> MTEYKIKATIEASVAKFKRQIDSAVKSVQRFKRVADQTKDVELNANDKKLQKTIKVAKKSLDAFSNKNVKAKLDASIQDLQQKILESNFELDKLNSKEASPEVKLQKQKLTKDIAEAENKLSELEKKRVNIDVNADNSKFNRVLKVSKASLEALNRSKAKAILDVDNSVANSKIKRTKEELKSIPNKTRSRLDVDTRLSIPTIYAFKKSLDALPNKKTTKVDVDTNGLKKVYAYIIKANDNFQRQMGNLANMFRVFGTVGSNMVGGLLTSSFSILIPVIASVVPVVFALLNAIKVLTGGVLALGGAVAIAGAGFVAFGAMAISAIKMLNDGTLQASSATNEYKKALDGVKSAWTDIIKQNQSAIFTTLANGLNTVKTAMQSLQPFFSGISRGMEEASQSVLKWAENSSVASRFFNMMNTTGVSVFNKLLSAAGGFGDGLVNVFTQLAPLFQWSADWLDRLGQSFSNWANSAAGENSITRFIEYTKTNLPIIGNIFKNVFAGINNLMNAFSGSSTGIFQSLEQMTAKFREWSEQVGQSQGFKDFVSYIQTNGPLIMQLIGNIARGLVAFATAMAPIASAVLRVAVA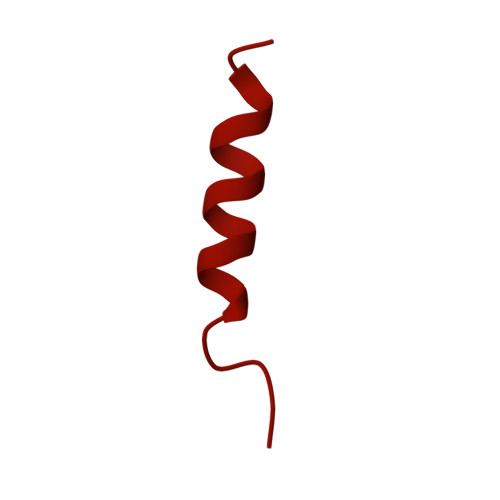ITGWIANLFEAHPATAQLVGVIITLVGAFRFLIAPILAVMDFLGPLAARLVALVTKFGWAKTGTLVLSKAMTSLKGPIKLVTAIFQLLFGKIGLIRNAITGLVTVFGILGGPITIVIGVIAALIAIFVLLWNKNEGFRNFIINAWNAIKTFMVNVWNVLKAVASVVWNAILTAITTAVSNVYNFIMIVWNQIVAYLQGLWNGIIAIATTVWNLLVTIITTVFTTIMTIVMTIWTAIWTFLSTIWNTIITIATTIWNLLVTVITTVFTTIMTIAMTIWNAIWTFLQTLWNTIVTVATKVWNAITTAISTALQAAWSFISNIWNTIWSFLSGILTTIWNKVVSIFTQVVSTISDKMSQAWNFIVTKGMQWVSTITSTLINFVNRVIQGFVNVVNKVSQGMTNAVNKIKSFIGDFVSAGADMIRGLIRGIGQMAGQLVDAAKNVAKKALDAAKSALGIHSPSREFMDVGMYSMLGFVKGIDNHSSKVIRNVSNVADKVVDAFQPTLNAPDISSITGNLSNLGGNINAQVQHTHSIETSPNMKTVKVEFDVNNDALTSIVNGRNAKRNSEYYL>[4x]QRVIPVYQVNNLEEICQLIIQAFEAGVDFQESADSFLLMLCLHHAYQGDYKLFLESGAVKYLEGHGFRFEVKKRDGVKRLEELLPAVSSGKNIKRTLAAMPEEETTEANAGQFLSFASLFLPKLVVGEKACLEKVQRQIQVHAEQGLIQYPTAWQSVGHMMVIFRLMRTNFLIK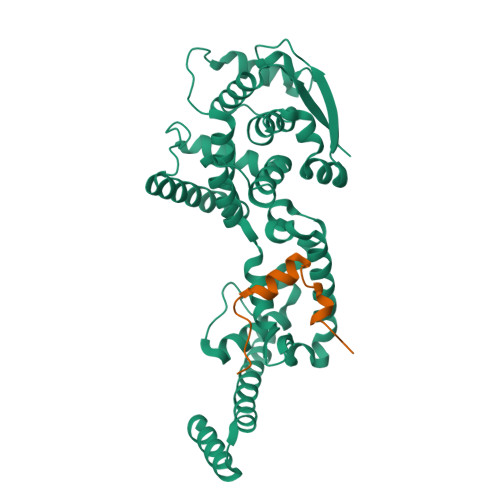FLLIHQGMHMVAGHDANDAVISNSVAQARFSGLLIVKTVLDHILQKTERGVRLHPLARTAKVKNEVNSFKAALSSLAKHGEYAPFARLLNLSGVNNLEHGLFPQLSAIALGVATAHGSTLAGVNVGEQYQQLREAATEAEKQLQQYAESRELDHLGLDDQEKKILMNFHQKKNE;>MPGPELSGWISEQLMTGRIPVSDIFCDI[4x]>GSHMGHWSQGLKISMQDPKMQVYKDEQVVVIKDKYPKARYQWLVLPWTSISSLKAVAREHLELLKHMHTVGEKVIVDFAGSSKLRFRLGYHAIPSMSHVHLHVISQDFDSPCLKNKKHWNSFNTEYFLESQAVIEMVQEAGRVTVRDGMPELLKLPLRCHECQQLLPSIP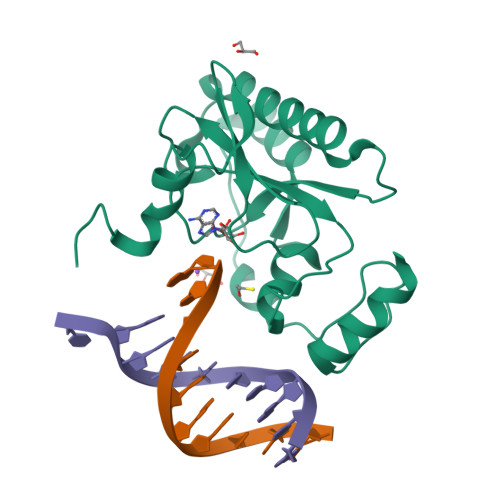QLKEHLRKHW[2x]> SEISRQEFQRRRQALVEQMQPGSAALIFAAPEVTRSADSEYPYRQNSDFWYFTGFNEPEAVLVLIKSDDTHNHSVLFNRVRDLTAEIWFGRRLGQDAAPEKLGVDRALAFSEINQQLYQLLNGLDVVYHAQGEYAYADVIVNSALEKLRKGSRQNLTAPATMIDWRPVVHEMRLFKSPEEIAVLRRAGEITAMAHTRAMEKCRPGMFEYHLEGEIHHEFNRHGARYPSYNTIVGSGENGCILHYTENECEMRDGDLVLIDAGCEYKGYAGDITRTFPVNGKFTQAQREI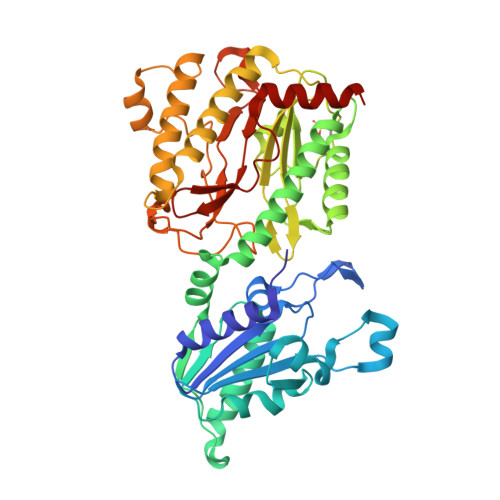YDIVLESLETSLRLYRPGTSILEVTGEVVRIMVSGLVKLGILKGDVDELIAQNAHRPFFMHGLSHWLGLDVHDVGVYGQDRSRILEPGMVLTVEPGLYIAPDAEVPEQYRGIGIRIEDDIVITETGNENLTASVVKKPEEIEALMVAARKQ>[4x]SNAIRPTIGQQMETGDQRFGDLVFRQLAPNVWQHTSYLDMPGFGAVASNGLIVRDGG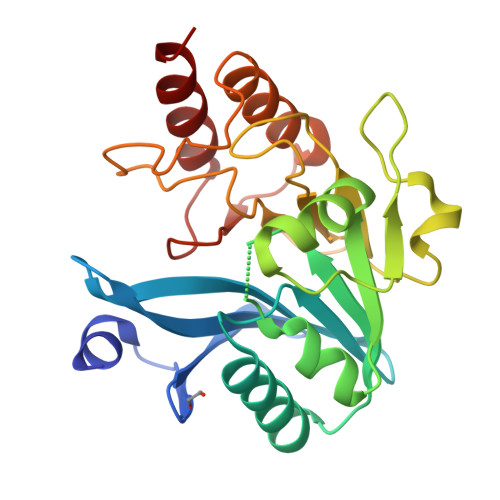RVLVVDTAWTDDQTAQILNWIKQEINLPVALAVVTHAHQDKMGGMDALHAAGIATYANALSNQLAPQEGMVAAQHSLTFAANGWVEPATAPNFGPLKVFYPGPGHTSDNITVGIDGTDIAFGGCLIKDSKAKSLGNLGAADTEHYAASARAFGAAFPKASMIVMSHSAPDSRAAITHTARMADKLR1-{6-[(1S)-1-hydroxyethyl]pyridin-2-yl}-6-{[4-(4-methylpiperazin-1-yl)phenyl]amino}-2-(prop-2-en-1-yl)-1,2-dihydro-3H-pyrazolo[3,4-d]pyrimidin-3-one | C26 H30 N8 O2 | 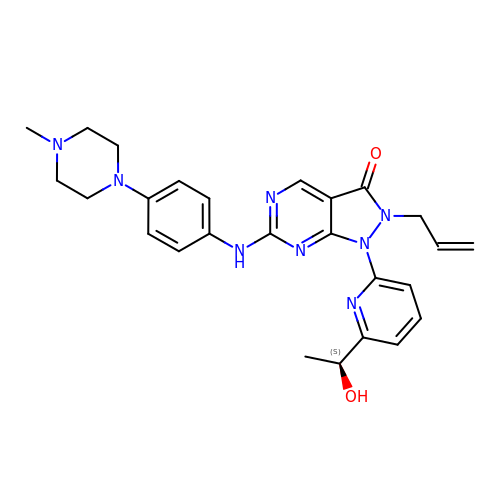FMCQFFXZPOWFBR-SFHVURJKSA-N5-BROMOVINYLDEOXYURIDINE | C11 H13 Br N2 O5 | 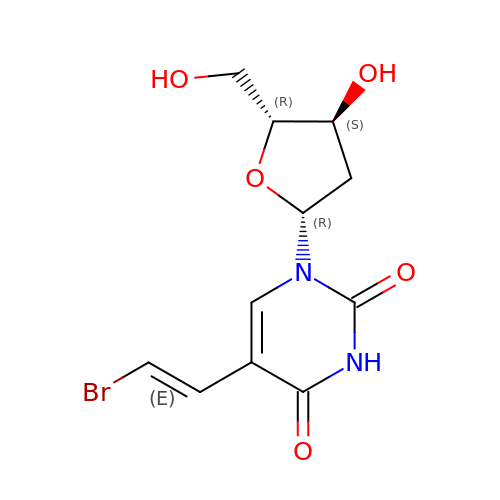ODZBBRURCPAEIQ-PIXDULNESA-N> MENSSKEDYKIQSFDLETQKLLKTALKDPGSVDLEKVSSVIVDQSLKDQVFSREAGRICYTIV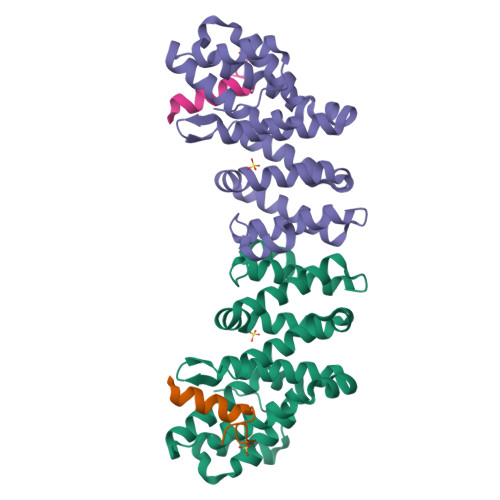QAEAKQTNGSVFRRNLLNRLQQEFKAREETRKRSTQEWVCLVSFICNIFDYLKVNNMPMVALVHPVYDCLFRLAQSDALKNEEEVDCLVLQLHRIGDQLEKMNVQLMDELFNLLRDGFLLQEDLSSMGRLLLLEILEFRAGGWKLSDTAQKYYYSEVTD;> PLGSMSRIKNWGDEVEEQEMRT6-{[(1R)-1-(3-hydroxyphenyl)ethyl]sulfanyl}-1-methyl-5-phenyl-1,5-dihydro-4H-pyrazolo[3,4-d]pyrimidin-4-one 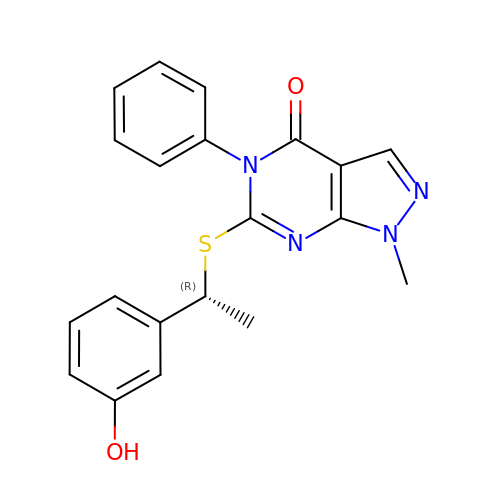| C20 H18 N4 O2 S | RTSMRTUJWIBZAN-CYBMUJFWSA-N> MTLIENLNSDKTFLENNQYTDEGVKVYEFIFGENYISSGGLEATKKILSDIELNENSKVLDIGSGLGGGCMYINEKYGAHTHGIDICSNIVNMANERVSGNNKIIFEANDILTKEFPENNFDLIYSRDAILHLSLENKNKLFQKCYKWLKPTGTLLITDYCATEKE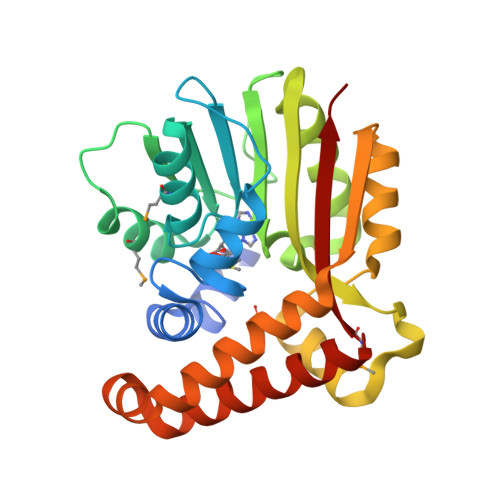NWDDEFKEYVKQRKYTLITVEEYADILTACNFKNVVSKDLSDYWNQLLEVEHKYLHENKEEFLKLFSEKKFISLDDGWSRKIKDSKRKMQRWGYFKATKN>UCUGGGCCAGGCAGG[3x];>[3x]CUUGCGCUC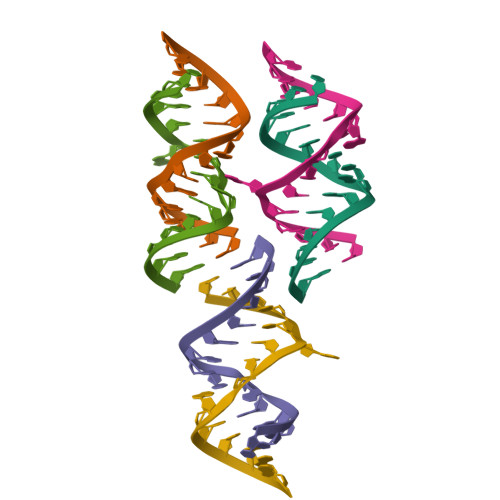AACCAGA> XGQLEEIAKQLEEIAWQLEEIAQ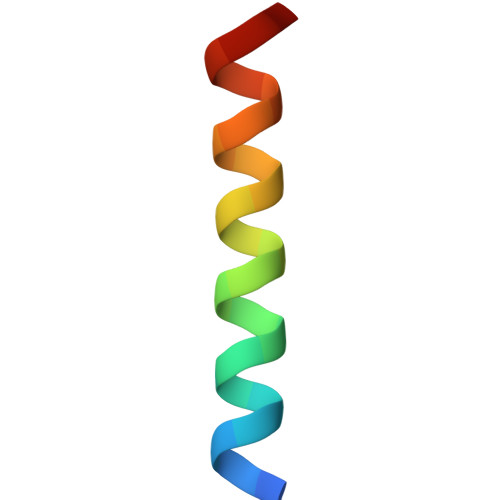GX> MGHHHHHHFDHSFSFDCQDKVILVVEDDYDIGD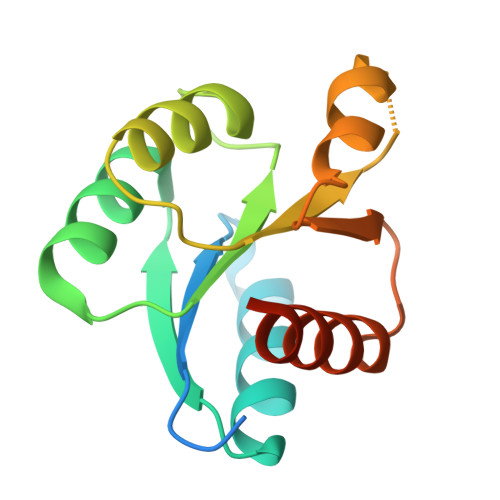IIENYLKREGMSVIRAMNGKQAIELHASQPIDLILLDIKLPELNGWEVLNKIRQKAQTPVIMLTALDQDIDKVMALRIGADDFVVKPFNPNEVIARVQAVLRRTQFANKATN> GRIRAVGIVGIERKLEEKRKETDKNISEAFEDLSKLMIKAKEMVELSKSIANKIKDKQGDITEDETIRFKSYLLSMGIANPVTRETYGSGTQYHMQLAKQLAGILQVPLEERGGIMSLTEVYCLVNRARGMELLSPE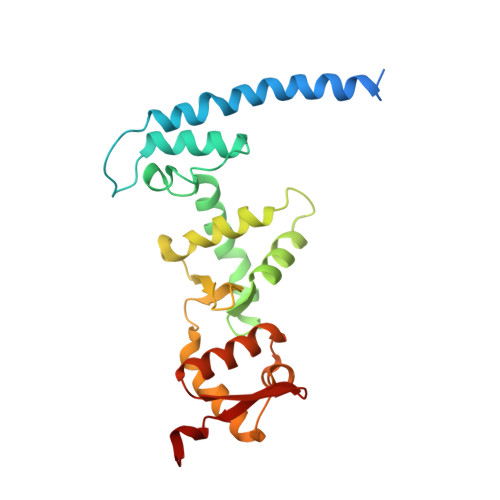DLVNACKMLEALKLPLRLRVFDSGVMVIELQSHKEEEMVASALETVSEKGSLTSEEFAKLVGMSVLLAKERLLLAEKMGHLCRDDSVEGLRFYPNLFMTQS>MAQSSNSTHEPLEVLKEETVNRHRAIVSVMEELEAVDWYDQRVDASTDPELTAILAHNRDEEKEAAAMTLEWLRRNDAKWAEHLRTYLFT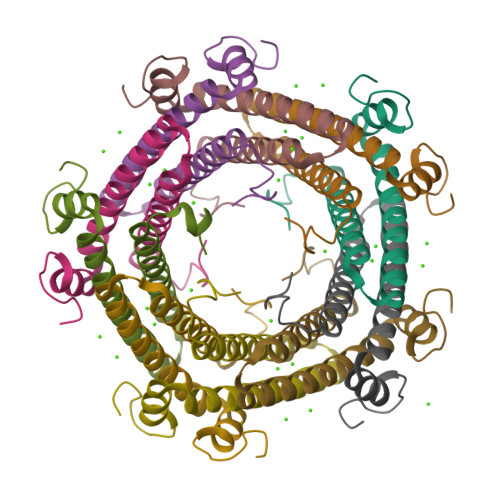EGPITAANSSSVDKLAAALEHHHHHH[30x]>MVLYFIGLGLYDERDITVKGLEIAKKCDYVFAEFYTSLMAGTTLGRIQKLIGKEIRVLSREDVELNFENIVLPLAKENDVAFLTPGDPLVATTHAELRI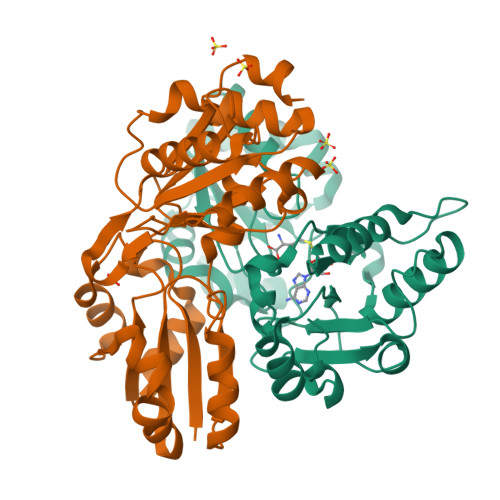RAKRAGVESYVIHAPSIYSAVGITGLHIYKFGKSATVMYPEGNWFPTSYYDVIKENAERGLHTLLFLDIKAEKRMYMTANEAMELLLKVEDMKKGGVFTDDTLVVVLARAGSLNPTIRAGYVKDLIREDFGDPPHILIVPGKLHIVEAEYLVEIAGAPREILRVNV[2x]>[2x]MENSLFNQEVQIPLTESYCGPCPKNWICYKNNCYQFFDESKNWYESQASCMSQNASLLKVYSKEDQDLLKLVKSYHWMGLVHIPTNGSWQWEDGSILSPNLLTIIEMQKGDCALYASSFKGYIENCSTPNTYICMQRTV;> MEPHSLRYNLTVLSWDGSVQSGFLTEVHLDGQPFLRCDRQKCRAKPQGQWAEDVLGNKTWDRETRDLTGNGKDLRMTLAHIKDQK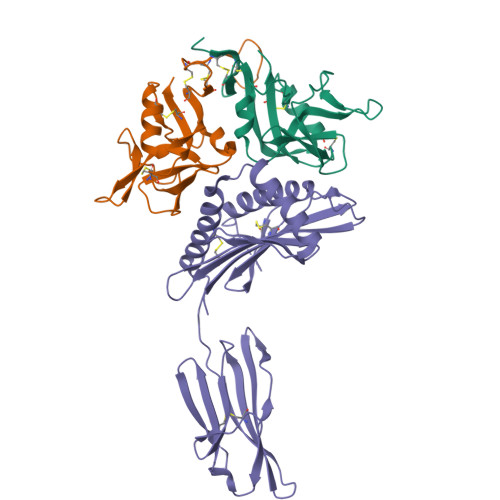EGLHSLQEIRVCEIHEDNSTRSSQHFYYDGELFLSQNLETKEWTMPQSSRAQTLAMNVRNFLKEDAMKTKTHYHAMRADCLQELRRYLKSGVILRRTVPPMVNVTRSEASEGNITVTCRASGFYPWNITLSWRQDGVSLSHDTQQWGDVLPDGNGTYQTWVATRICQGEEQRFTCYMEHSGNHSTHPVPS>MSLLSDLCNLNLSESTEKIIAEYIWIGGSGMDLRSKARTLNAPVSDPSKLPQWNYDGSSTGQAPGEDSEVILYPQAIYKDPFRRGNNILVMCDAYTPGGEPIPTNKRFDAAKIFSHPDVVAEEPWYGIEQEYTLLQKEVKWPIGWPVGGYPGPQGPYYCGIGADKAFGRDIVDAHYKACLYAGINISGINGEVMPGQWEFQVGPSVGISSGDQLWMARYILERITEIAGVVVSFDPKPIEGDWNGAGAHTNYSTKSMRSDGGFEVIKKAIEKLGLKHREHIAAYGEGNERRLTGKHETADINTFLWGVANRGASIRVGRDTEKAGK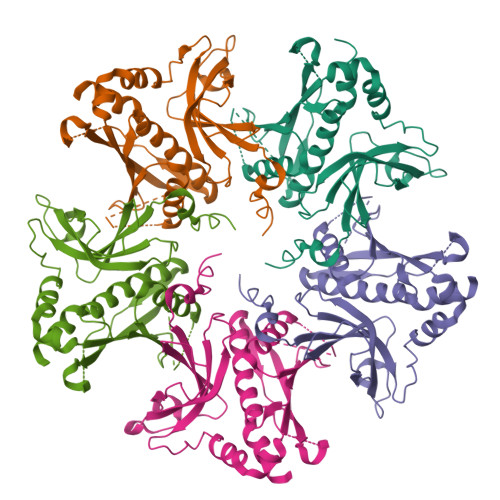GYFEDRRPASNMDPYIVTSMIANTTILWKP[5x]> LFLAQEIIRKKRDGHALSDEEIRFFINGIRDNTISEGQIAALAMTIFFHDMTMPERVSLTMAMRDSGTVLDWKSLHLNGPIVDKHSTGGVGDVTSLMLGPMVAACGGYIPMISGRGLGHTGGTLDKLESIPGFDIFPDDNRFREIIKDVGVAIIGQTSSLAPADKRFYATRDITATVDSIPLITASILAKKLAEGLDALVMDVKVGSGAFMPTYELSEALAEAIVGVANGAGVRTTALLTDMNQVLASSAGNAVEVREAVQFLTGEYRNPRLFDVTMALCVEMLISGKLAKDDAEARAKLQAVLDNGKAAEVFGRMVAAQKGPTDFVENYAKYLPTAM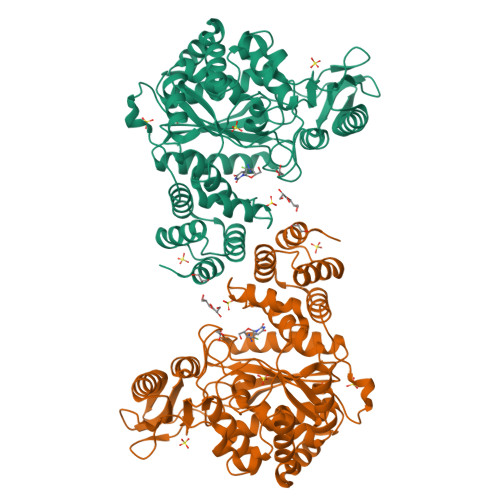LTKAVYADTEGFVSEMDTRALGMAVVAMGGGRRQASDTIDYSVGFTDMARLGDQVDGQRPLAVIHAKDENNWQEAAKAVKAAIKLADKAPESTPTVYRRISE> HGMSQPACTARRRTRVLILGVNGFIGNHLTERLLREDHYEVYGLDIGSDAISRFLNHPHFHFVEGDISIHSEWIEYHVKKCDVVLPLVAIATPIEYTRNPLRVFELDFEENLRIIRYCVKYRKRIIFPSTSEVYGMCSDKYFDEDHSNLIVGPVNKPRWIYSVSKQLLDRVIWAYGEKEGLQFTLFRPFNWMGPRLDNLNAARIGSSRAITQLILNLVEGSPIKLIDGGKQKRCFTDIRDGIEALYRIIENAG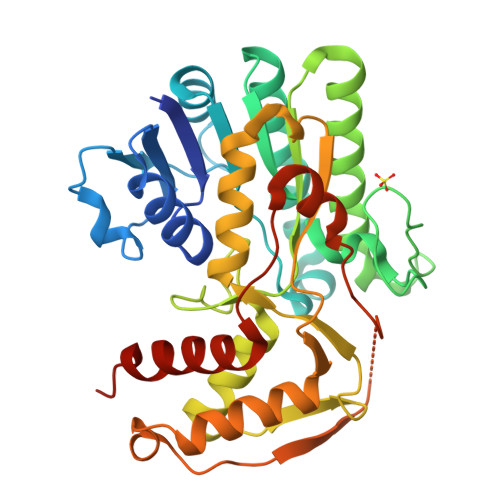NRCDGEIINIGNPENEASIEELGEMLLASFEKHPLRHHFPPFAGFRVVESSSYYGKGYQDVEHRKPSIRNAHRCLDWEPKIDMQETIDETLDFFLRTVDLTDKPS>[20x]TPDCVTGKVEYTKYN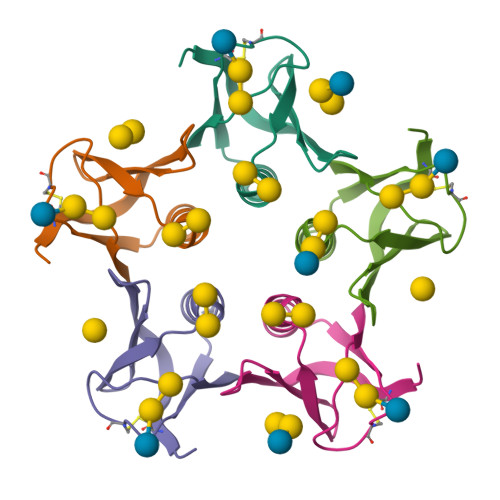DDDTFTVKVGDKELFTNRWNLQSLLLSAQITGMTVTIKTNACHNGGGFSEVIFR>NGQGSDPAVTYYRLEEVAKRNTSEETWMVLHGRVYDLTRFLSEHPGGEEVLREQAGADATESFEDVGHSPDAREMSKQYYIGDVHPNDL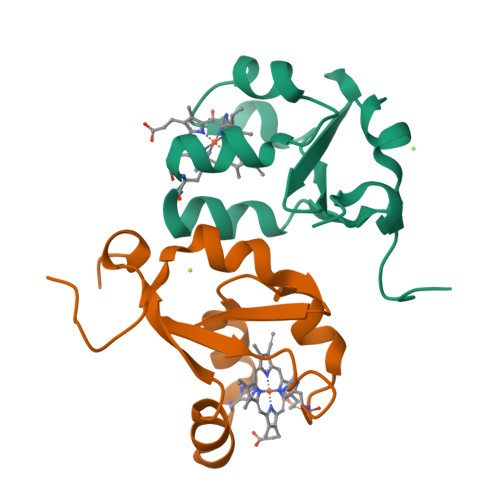KPK[4x]> MSQIPASEQETLVRPKPLLLKLLKSVGAQKDTYTMKEVLFYLGQYI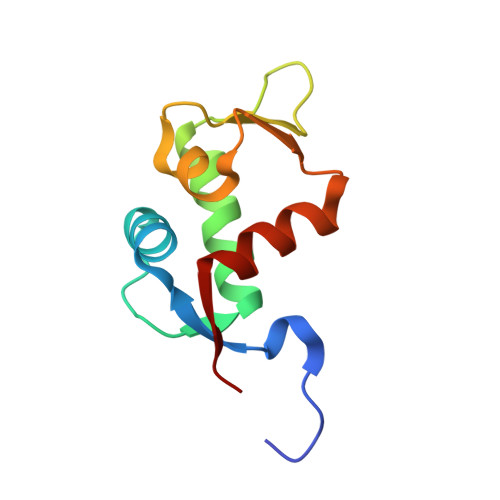MTKRLYDEKQQHIVYCSNDLLGDLFGVPSFSVKEHRKIYTMIYRNLVVVN> MKYSQCLKGEVVMIPALAKKILHVTVGTLLVSSAASMMVYLNSM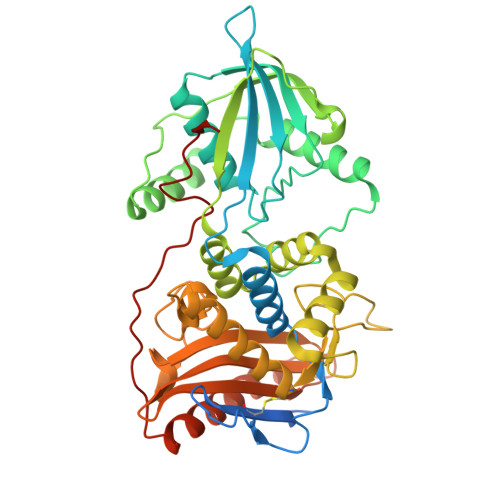CHMAANSKTQQIQGDDNKDDKFPLASISKVVTTLWAVDRLGPDYRFKTKLHVTPTANGSYDIHIEGSRDPLFGRNMSYFLISELNRMKITKIEKLTFDENFLLAWLAEEKPMIGGTTPKYDTVEQQASIVRATLTSSFATAISPGYYTILKTKAARIGVQMSNRPKIDVRTISFVKKAEFQKNEKSTTMVLMSAPLKTILKRMNNQSNNYIADNLYWNLGGTEAFNAYIAGKMQADTSDIEFHNGSGNNEGSVAKPVYNEATCEMMIKVLYSLDKSLSAKGYDLSDVMAVAAKDKASTVGSYGGVMAGSTTAKTGSVNKAKTLMGSVSTKNGEIYFAVLMHTDYDKSRSDWGVASQQIKNKVSQLINQNGGPKAIKYTEQLPLPFDKYSYLTKANTITTEKK>[3x]MGGSHHHHHHGMASWSHPQFEKGGHHHHHHGGSGENLYFQGGSGPKFNETADKYLKSGSAEAELIILQYIQQDRVSEDDEEWVYNLLEKANNPYIKLNALLWLSAKRKYLTQLSKLWGISENELKSLSQQQPKIGLFPAVDSRKNAFLAKVFVYKLKSEEPIALAILGDKIENFSYLAQLGKQNCLIGFNKNIQGNSWQLAVLATLLVKDEKIISKIAYSGIVLPSGEIITAEEIEYKKRCCQNLVHRIKKIEQLDAWLNTETIPLPVIQYQGEENELKRWQKAMEQKVQEKFSWFSYELLEDFYGITNSDLAIFGNGILPFEANAWQKLLQEQVKDKFKLLEDKVMPKKVLWFYAGQISTLQLGIGALFGFKRAVSILQMEFSNTTYHEVFILYGKENARQLKNVSVKKEDYQYIQSELLINEPHKNELGFIIYLGSHNPIGEAKAYCQKQLQINNFLII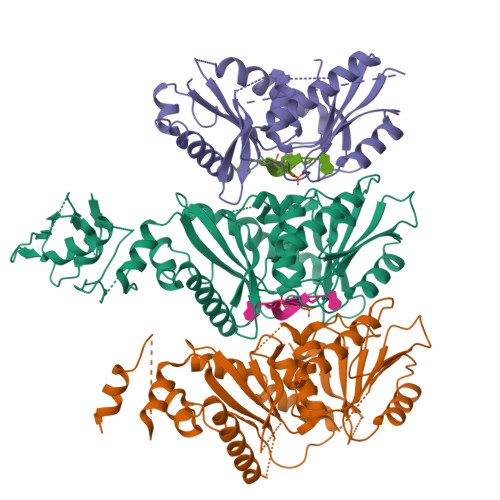QARENQGVMETSQNWLPYLQEINSALNTARQEYHWERIHLFQTAPTALCMALGIAVGHFLPVDVYHYQFNAEEPKYRCVFSLDKMLNL>MAVKISGVLKDGTGKPVQNCTIQLKARRNSTTVVVNTVGSENPDEAGRYSMDVEYGQYSVILQVDGFPPS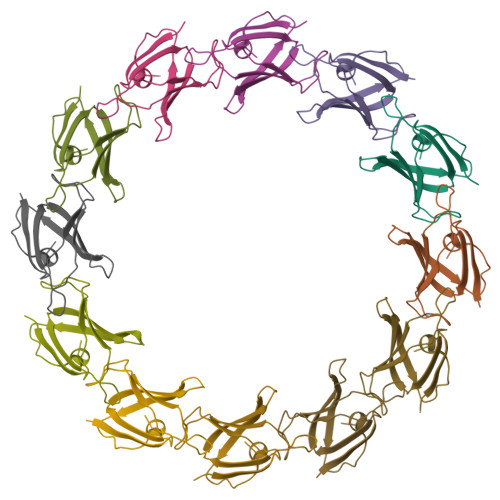HAGTITVYEDSQPGTLNDFLCAMT[12x]p-nitrophenylboronic acid | C6 H6 B N O4 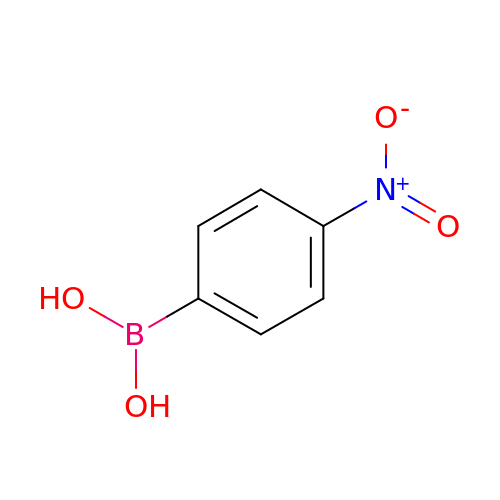| NSFJAFZHYOAMHL-UHFFFAOYSA-N3-methyl-1-(5-oxohexyl)-7-propyl-3,7-dihydro-1H-purine-2,6-dione 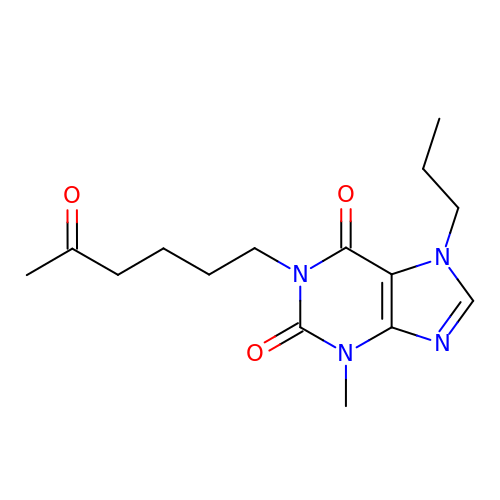| C15 H22 N4 O3 | RBQOQRRFDPXAGN-UHFFFAOYSA-N>[4x]AATATLPTTASSSTAVASSQLDQLANFAYNVTTDSVAGGSESKRGGCTLQNLRVRRDWRAFSKTQKKDYINSVLCLQKLPSRTPAHLAPGARTRYDDFVATHINQTQIIHYTGTFLAWHRYFIYEFEQALRDECSYTGDYPYWNWGADADNMEKSQVFDGSETSMSGNGEYIPNQ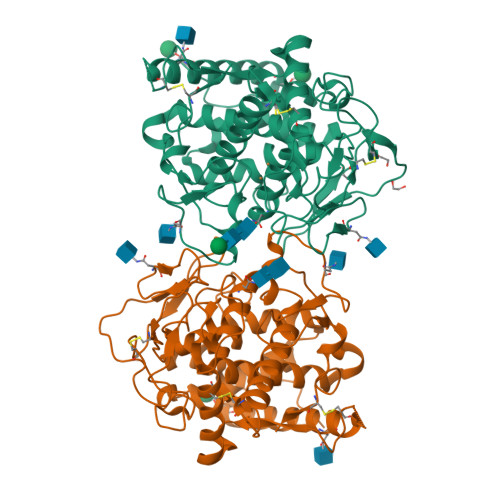GDIKLLLGNYPAIDLPPGSGGGCVTSGPFKDYKLNLGPAALSLPGGNMTAAANPLTYNPRCMKRSLTTEILQRYNTFPKIVELILDSDDIWDFQMTMQGVPGSGSIGVHGGGHYSMGGDPGRDVYVSPGDTAFWLHHGMIDRVWWIWQNLDLRKRQNAISGTGTFMNNPASPNTTLDTVIDLGYANGGPIAMRDLMSTTAGPFCYVYL> MLLIYIML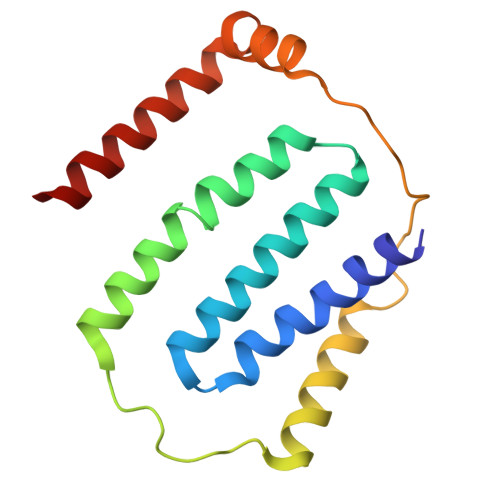SNIVVLALSVVLTSSPFMALMYSILLYLNVQTILWSLGYDFMALIYALVYVGALAVLFLFVVMMVRIQVSTLSTKTIQSVLSWLAIILIFSYGDVSFSFPCGAESLLNFGTQLYSSCSDLTLLNSLALTIALFGSLV> MGILFTPENDDPYANISSHKAFTHAYLSTVTADFGGDNFLTCPLGILFTLGILLGSGGAQGRTGYQIGKTMRLKSTSSSWNSSEAQQEMKSLYQELNNSLTSEKTFLNEKEENVVRISTGIFVEKTYEVERRFNESIANDSEGELKQVDFSNRTSATVDINDWVDQQSNGLLEKFFTDDIPDDTAMILVNVFYFRDFWQSPFEPHYTRKEDFYISPDRQITVDMMTQEGVMKYG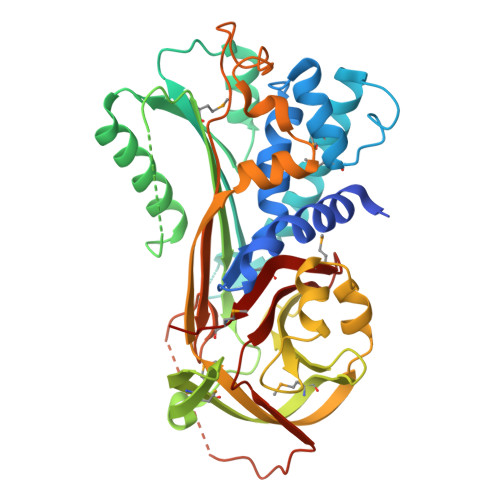KFEDEGFEIVSKPLNNTRFTFVIVLPLEKWSLNGATELLNGNKVLSEYVKNLKETTVSLRLPKFTLKNTLDLVPTLKSIGVVDLFDPVKSDLSGITPNPNLYVNEFIQTNVLKLNESGIEATTVTSPIFVPFSAIIPEVDFHVTHPFICFIYDQQLTMPIMAAKVMNPVLQS> MNSQNSQIQPQARYILPSFIEHSSFGVKESNPYNKLFEERIIFLGVQVDDASANDIMAQLLVLESLDPDRDITMYINSPGGGFTSLMAIYDTMQYVRADIQTVCLGQAASAAAVLLAAGTPGKRMALPNARVLIHQPSLSGVIQGQFSDLEIQAAEIERMRTLMETTLARHTGKDAG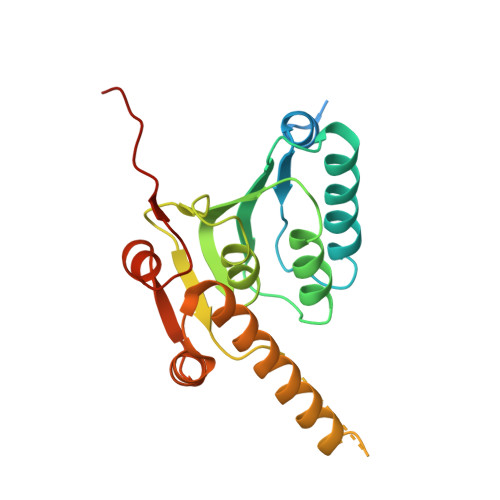VIRKDTDRDKILTAEEAKDYGIIDTVLEYRKLSAQTA Furthermore, in situ X-ray-driven generation of haem intermediates in crystals of the dye-decolourizing-type peroxidase A (DtpA) from Streptomyces lividans is described. We describe the use of online UV–visible spectroscopy to monitor the X-ray-generated formation of an oxyferrous complex of the dye-decolorizing-type peroxidase A (DtpA) from Streptomyces lividans, allowing its structural characterization. High-resolution crystal structures determined using synchrotron radiation are central to our understanding of haem-protein function. The correct assignment of crystal structures to the correct protein redox and ligand states is essential to avoid the misinterpretation of structural data. This is a particular concern for haem proteins, which can occupy a wide range of redox states and are exquisitely sensitive to becoming reduced by solvated electrons generated from interactions of X-rays with water molecules in the crystal.

A further high-resolution crystal structure was determined using a second dose of 0.99 MGy (an accumulated dose of 1.98 MGy) to a resolution of 1.49 Å. One O atom is ligated to the haem Fe at adistances of 2.3 and 2.1 Å in monomers A and B, respectively, as well as making a polar interaction with the distal pocket residue Arg369. Therefore, we conclude from the structure and the spectroscopic data that the haem is in a six-coordinate ferrous state with an O atom bound (oxy­ferrous). Examination of the electron-density maps and structures for the two successive DtpA structures (with accumulated doses of 0.99 and 1.98 MGy, respectively) revealed no substantial differences in coordinates or B factors and no appreciable signs of specific radiation damage beyond the haem pocket. For the present crystal the 0.99 MGy initial structure has two molecules in the crystallo­graphic asymmetric unit, denoted here as A and B, and has been determined to 1.45 Å resolution. See Table 2 for crystallographic data-collection statistics and refinement details and Table 3 for geometrical values for the haem site of the oxyferrous DtpA structure. The structures allowed the assignment of 100 K spectra to either a diatomic (oxygen) or monatomic (compound III) state, while the spectra allowed X-ray and ligand-soaking effects to be precisely monitored.

>ATPLTSLGSEQAMFHGKHQPGITTPMQARGHLVAFDLAAGAGRKEAAALLRRWSDTARRLMAGEPAGSRDTDVARDAGPSSLTVTFGFGHSFFGRTGLEKQRPVALDPLPDFSSDHLDKNRSNGDLWVQIGADDALVAFHALRAIQRDAGAAARVRWQMNGFNRSPGATAHPMTARNLMGQVDGTRNPKPGEADFDRRIFVPEEPEAGKGGPAWMANGSYVVVRRIRMLLDDWEELSLKAQEDVIGRRKSDGAPLSGGSGATESTEMDLEKTDGSGELVVPINAHARITRPDQNGGAAMVRRPFSYHDGFDADGVPDAGLLFVCWQADPLRGFVPVQRKLDRGDALSQFIRHEASGLFAVPGGAAEGEYVGQRLLE[2x]>[6x]GPGSMAKGNGLLYGKRGLILGLANNRSIAWGIAKTASSAGAELAFTYQGEAMKKRVEPLAEEVKGFVCGHCDVSDSASIDAVFNTIEKKWGKLDFLVHAIGFSDKEELSGRYVDISESNFMMTMNISVYSLTALT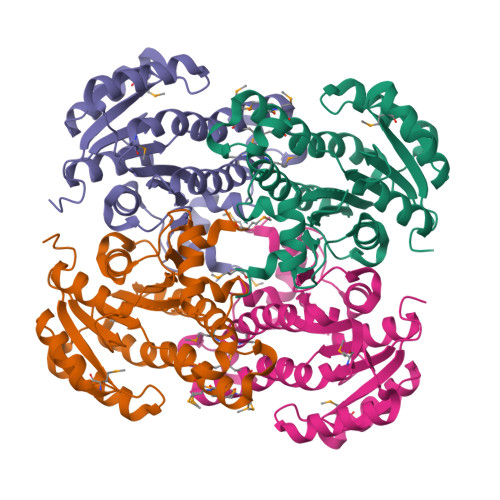KRAEKLMSDGGSILTLTYYGAEKVVPNYNVMGVAKAALEASVKYLAVDLGPKHIRVNAISAGPIKTLAASGIGDFRYILKWNEYNAPLRRTVTIEEVGDSALYLLSDLSRSVTGEVHHVDSGYNIIGMKAVDAPDISVVKE>MERTGFLEYVLNYVKKGVELGGFPEDFYKILSRPRRVLIVNIPVRLDGGGFEVFEGYRVQHCDVLGPYKGGVRFHPEVTLADDVALAILMTLKNSLAGLPYGGAKGAVRVDPKKLSQRELEELSRGYARAIAPLIGDVVDIPAPDVGTNAQIMAWMVDEYSKIKGYNVPGVFTSKPPELWGNPVREYATGFGVAVATREMAKKLWGGIEGKTVAIQGMGNVGRWTAYWLEKMGAKVIAVSDINGVAYRKEGLNVELIQKNKGLTGPALVELFTTKDNAEFVKNPDAIFKLDVDIFVPAAIENVIRGDNAGLVKARLVVEGANGPTTPEAERILYERGVVVVPDILANAGGVIMSYLEWVENLQWYIWDEEETRKRLENIMVNNVERVYKRWQ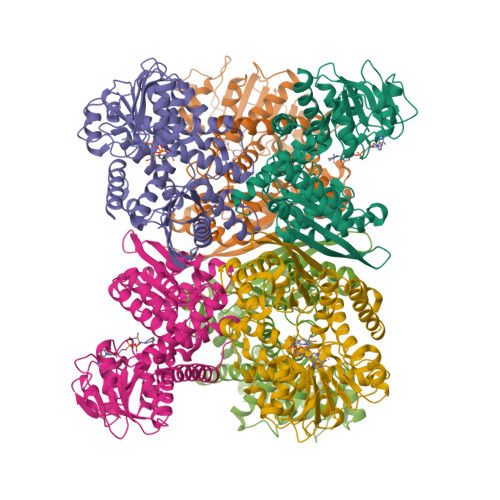REKGWTMRDAAIVTALERIYNAMKIRGWI[6x]2-oxidanylidene-N-piperidin-4-yl-1,3-dihydroindole-5-carboxamide 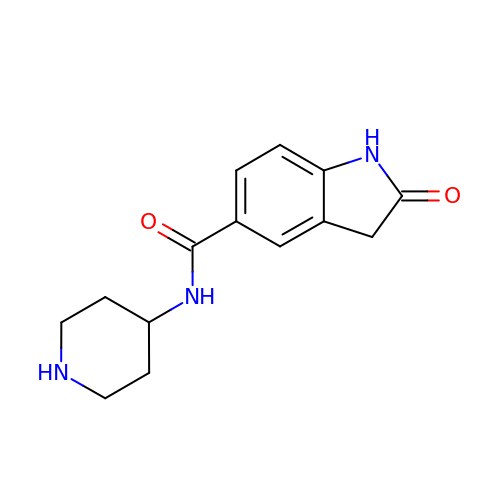| C14 H17 N3 O2 | SWMKOYKJOHHEQD-UHFFFAOYSA-N> SNAMSKLDRIRHFLNENKSGLAIVSDPVTVNYLTGFDCDPHERQMFLFVYENREPALFVPALEVARASSVLDFPVFGYVDSENPWQKIKAGLASTDIPIIYAEFDNLNVTKFQGLQTVFEGRFENLTPFIHKM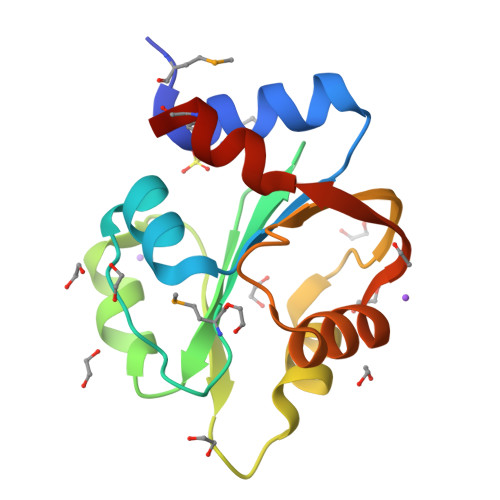RVIK>[4x]GMDAKARNCLLQHREALEKDIKTS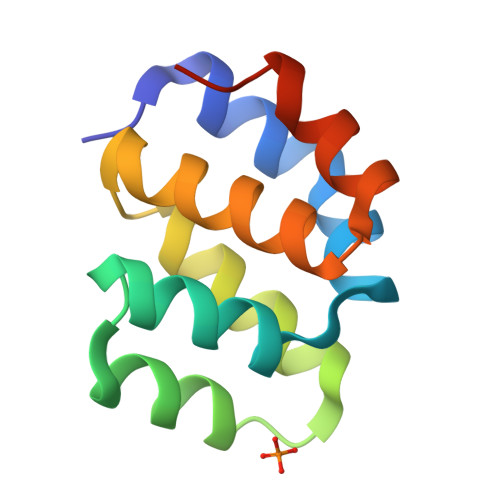YIMDHMISDGFLTISEEEKVRNEPTQQQRAAMLIKMILKKDNDSYVSFYNALLHEGYKDLAALLHDGIPVVSSS> PAPGDKFELSGWSLSVPVDSDNDGKADQIKEKTLAAGYRNSDFFTLSDAGGMVFKAPISGAKTSKNTTYTRSELREMLRKGDTSIATQGVSRNNWVLSSAPLSEQKKAGGVDGTLEATLSVDHVTTTGVNWQVGRVIIGQIHANNDEPIRLYYRKLPHHQKGSVYFAHEPRKGFGDEQWYEMIGTLQPSHGNQTAAPTEPEAGIALGETFSYRIDATGNKLTVTLMREGRPDVVKTVDMSKSGYSEAGQYLYFKAGVYNQNKTGKPDDYVQATFYRLKATHG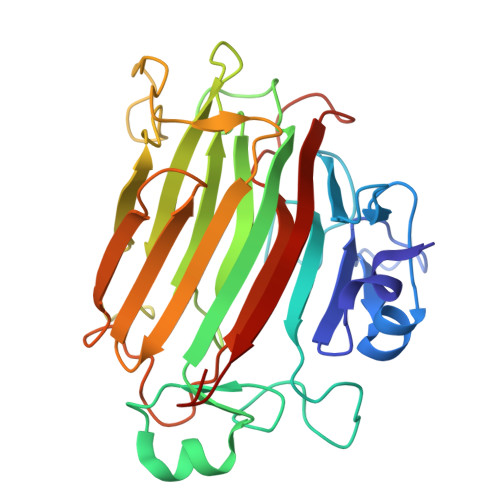AQR>GMTSSFTDYCKFFNRILSEVQETQEQAIIKGAHLVSEAVMNGGRFYVFGSGHSHMIAEEIYNRAGGLALVTAILPPELMLHERPNKSTYLERIEGLSKSYLKLHQVTNKDVIMIISNSGRNTVPVEMAIESRNIGAKVIAMTSMKHSQKVTSRHKSGKKLYEYADVVLDNGAPVGDAGFQIANSEIYSGATSDS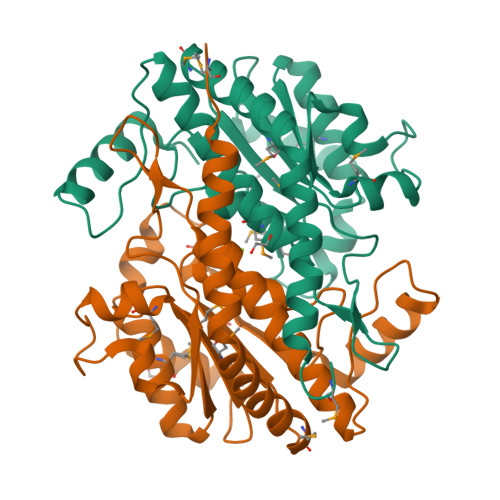IGCFLAQALIVETLHLLVQQGFEPPVFKSSNVDGADLYNDKIFNEYVKW[4x]>[3x]AHNNENVSGISAYLLGLIISDGGLYKLKYKGNRSEYRVVITQKSENLIKQHIAPLMQFLIDELNVKSKIQIVKGDTRYELRVSSKKLYYYFANMLERIRLFNMREQIAFIKGL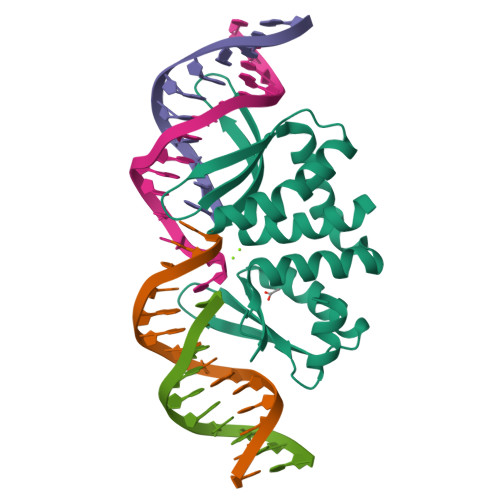YVAEGDKTLKRLRIWNKNKALLEIVSRWLNNLGVRNTIHLDDHRHGVYVLNISLRDRIKFVHTILSSHLNPLPPEAAALEHHHHHH> MTSPAKFKKDKEIIAEYDTQVKEIRAQLTEQMKCLDQQCELRVQLLQDLQDFFRKKAEIEMDYSRNLEKLAERFLAKTRSTKDQQFKKDQNVLSPVNCWNLLLNQVKRESRDHTTLSDIYLNNIIPRFVQVSEDSGRLFKKSKEVGQQLQDDLMKVLNELYSVMKTYHMYNADSISAQSKLKEAEKQEEKQIGKSVKQEDRQTPRSPDSTANVRIEEKHVRRSSVKKIEKMKEKRQAKYTENKLKAIKARNEYLLALEATNASVFKYYIHDLSDLIDQCCDLGYHASLNRALRTFLSAELNLEQSKHEGLDAIENAVENLDATSDKQRLMEMYNNVFCPPMKFEFQPHMGDMASQLCAQQP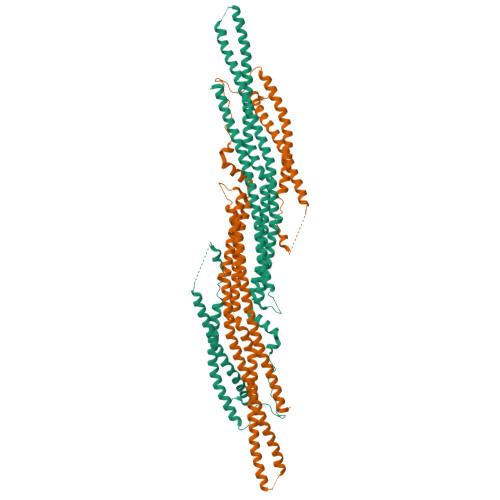VQSELVQRCQQLQSRLSTLKIENEEVKKTMEATLQTIQDIVTVEDFDVSDCFQYSNSMESVKSTVSETFMSKPSIAKRRANQQETEQFYFTKMKEYLEGRNLITKLQAKHDLLQKTLGESQRT>MISSFEVRKATIDDYFELRNLICDVTRCTETLSREQAEERFRYNTYHPYCLVDTENGRIVGYAGFYIIPHLGRKNDSRIEHVIISKEYRNRGLGRLLCKQIIEDAKNKFNCGRIDLTVES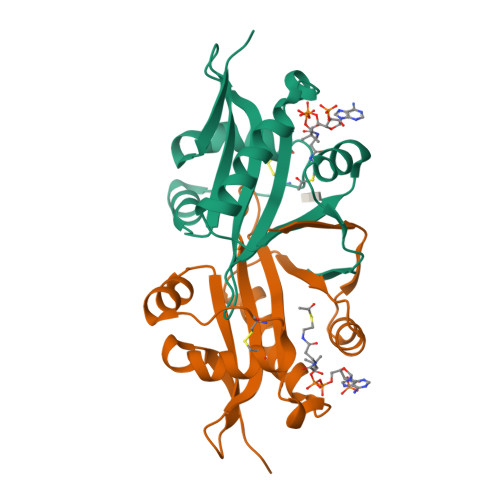HIAKKLYSSLEFEKVNTEVMRNSFLDLTPKSD[2x]>[2x]MKHLTEEQKLTLDMVRDVATREIAPRALELDEKSLFPEYARDLFAKLGLLNPLLPAAYGGTEMGVLTLALILEELGRVCASTALLLIAQTDGMLPIIHGGSPELKERYLRRFAGESTLLTALAATEPAAGSDLLAMKTRAVRQGDKYVINGQKCFITNGSVADVIVVYAYTDPEKGSKGISAFVVEKGTPGLVYGRNESKMGMR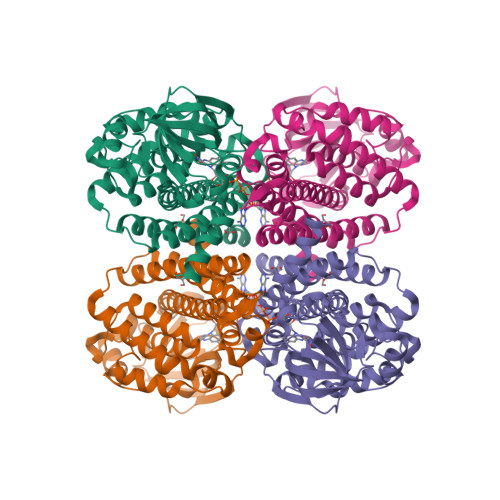GSINSELFFENMEVPAENIIGAEGTGFANLMQTLSTNRVFCAAQAVGIAQGALDIAVRHTQDRVQFGKPIAHLAPVQFMVADMATAVEASRLLTRKAAELLDDGDKKAVLYGSMAKTMASDTAMRVTTDAVQVLGGSGYMKENGVERMMRDAKLTQIYTGTNQITRMVTGRALLFPKGELNSKLEGKPIPNPLLGLDSTRTGHHHHHH> MYYESLTKQYPVSKTIRNELIPIGKTLDNIRQNNILESDVKRKQNYEHVKGILDEYHKQLINEALDNCTLPSLKIAAEIYLKNQKEVSDREDFNKTQDLLRKEVVEKLKAHENFTKIGKKDILDLLEKLPSISEDDYNALESFRNFYTYFTSYNKVRENLYSDKEKSSTVAYRLINENFPKFLDNVKSYRFVKTAGILADGLGEEEQDSLFIVETFNKTLTQDGIDTYNSQVGKINSSINLYNQKNQKANGFRKIPKMKMLYKQILSDREESFIDEFQSDEVLIDNVESYGSVLIESLKSSKVSAFFDALRESKGKNVYVKNDLAKTAMSNIVFENWRTFDDLLNQEYDLANENKKKDDKYFEKRQKELKKNKSYSLEHLCNLSEDSCNLIENYIHQISDDIENIIINNETFLRIVINEHDRSRKLAKNRKAVKAIKDFLDSIKVLERELKLINSSGQELEKDLIVYSAHEELLVELKQVDSLYNMTRNYLTKKPFSTEKVKLNFNRSTLLNGWDRNKETDNLGVLLLKDGKYYLGIMNTSANKAFVNPPVAKTEKVFKKVDYKLLPVPNQMLPKVFFAKSNIDFYNPSSEIYSNYKKGTHKKGNMFSLEDCHNLIDFFKESISKHEDWSKFGFKFSDTASYNDISEFYREVEKQGYKLTYTDI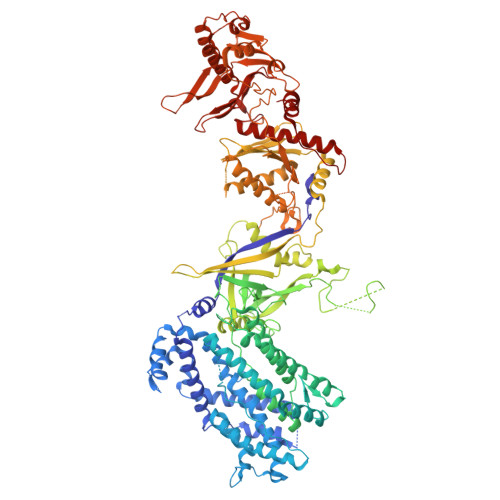DETYINDLIERNELYLFQIYNKDFSMYSKGKLNLHTLYFMMLFDQRNIDDVVYKLNGEAEVFYRPASISEDELIIHKAGEEIKNKNPNRARTKETSTFSYDIVKDKRYSKDKFTLHIPITMNFGVDEVKRFNDAVNSAIRIDENVNVIGIDRGERNLLYVVVIDSKGNILEQISLNSIINKEYDIETDYHALLDEREGGRDKARKDWNTVENIRDLKAGYLSQVVNVVAKLVLKYNAIICLEDLNFGFKRGRQKVEKQVYQKFEKMLIDKLNYLVIDKSREQTSPKELGGALNALQLTSKFKSFKELGKQSGVIYYVPAYLTSKIDPTTGFANLFYMKCENVEKSKRFFDGFDFIRFNALENVFEFGFDYRSFTQRACGINSKWTVCTNGERIIKYRNPDKNNMFDEKVVVVTDEMKNLFEQYKIPYEDGRNVKDMIISNEEAEFYRRLYRLLQQTLQMRNSTSDGTRDYIISPVKNKREAYFNSELSDGSVPKDADANGAYNIARKGLWVLEQIRQKSEGEKINLAMTNAEWLEYAQTHLL Aspartate ammonia lyases catalyze the reversible amination of fumarate to l-aspartate. Furthermore, a conserved flexible loop, named SS-loop, that contains a two serine signature sequence plays an important role in substrate binding and catalysis. One of the serines acts as a general base in the deamination reaction by abstracting a proton from the Cβ atom of the substrate, forming an enolate anion intermediate. For this, the SS-loop changes from an open conformation in the absence of substrate to a closed conformation that covers the active site in the presence of substrate.

b The variant of AspB carrying the AspB-A1 pocket (T187I+M321I+K324M+N326C) and the loop mutations A422S+Y429D were used further and relabeled AspB-6x. To rationalize the effect of mutations that allowed for β-alanine synthesis, crystal structures of variants AspB-6x and CcAsp-6x were determined to 1.9 and 3.1 Å resolution, respectively. Both variants were crystallized in an apo state: cocrystallization and crystal soaking experiments with acrylic acid, ammonia, or β-alanine did not yield a structure with a bound ligand. While the wild-type AspB crystal structure contains both open and closed SS-loops, unliganded AspB-6x and CcAsp-6x adopted the typical closed conformation observed previously only in the liganded active sites of wild-type AspB. In AspB-6x, the introduced Ile321 interacts with Val193, while Met324 makes hydrophobic contacts with Ala192, Gln190, and the mutated Ile187. Additional hydrophobic contacts are formed between Cys326 and Val328. Thus, the mutations that remove the charged binding pocket for the α-carboxylate group of aspartate may also have a stabilizing effect on the closed SS-loop conformation. In contrast, the activity-enhancing A422S and Y429D mutations that were designed to promote the closed conformation of the SS-loop in AspB-6x are positioned in helix α16 of the small C-terminal domain of an adjacent subunit. In the crystal structure of wild-type AspB, the open conformation of the SS-loop at unliganded active sites is stabilized via hydrophobic interactions with C-terminal domain residues Ile406, Tyr418, Ala421, Ala422, Ala425, and Tyr429.17 Mutations A422S and Y429D disrupt this hydrophobic cluster and thus will destabilize the open-loop conformation and shift the equilibrium toward the closed-loop conformation.

>[2x]MNTDVRIEKDFLGEKEIPKDAYYGVQTIRATENFPITGYRIHPELIKSLGIVKKSAALANMEVGLLDKEVGQYIVKAADEVIEGKWNDQFIVDPIQGGAGTSINMNANEVIANRALELMGEEKGNYSKISPNSHVNMSQSTNDAFPTATHIAVLSLLNQLIETTKYMQQEFMKKADEFAGVIKMGRIHLQDAVPILLGQEFEAYARVIARDIERIANTRNNLYDINMGATAVGTGLNADPEYISIVTEHLAKFSGHPLRSAQHLVDATQNTDCYTEVSSALKVCMINMSKIANDLRLMASGPRAGLSEIVLPARQPGSSIIPGMVCPVMPEVMNQVAFQVFGNDLTITSASEAGQFELNVMEPVLFFNLIQSISIMTNVFKSFTENCLKGIKANEERMKEYVEKSIGIITAINPHVGYETASKLAREADLTGESIRELCIKYGVLTEEQLNEILNPYEMIHPGIAGRK> MGKYFGTDGVRGVANSELTPELAFKVGRFGGYVLTKDKQRPKVLIGRDTRISGHMLEGALVAGLLSIGAEVMRLGVISTPGVSYLTKAMDAEAGVMISASHNPVQDNGIKFFGGDGFKLSDEQEAEIERLMDEPEDKLPRPVGADLGLVNDYFEGGQKYLQFLKQTADEDFTGIHVALDCANGATSSLATHLFADLDADVSTMGTSPNGLNINDGVGSTHPEALSAFVKEKNADLGLAFDGDGDRLIAVDEKGNIVDGDQIMYICSKHLKSEGRLKDDTVVSTVMSNLGFYKALEKEGIKSVQTAVGD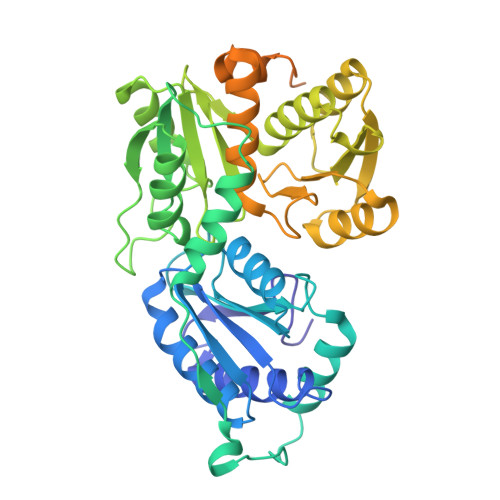RYVVEAMKKDGYNVGGEQSGHLIFLDYNTTGDGLLSAIMLMNTLKATGKPLSELAAEMQKFPQLLVNVRVTDKYKVEENEKVKAVISEVEKEMNGDGRILVRPSGTEPLVRVMAEAKTKELCDEYVNRIVEVVRSEMGLELVPRGSSGLEHHHHHH> MAAPFDKSKNVAQSIDQLIGQTPALYLNKLNNTKAKVVLKMECENPMASVKDRLGFAIYDKAEKEGKLIPGKSIVVESSSGN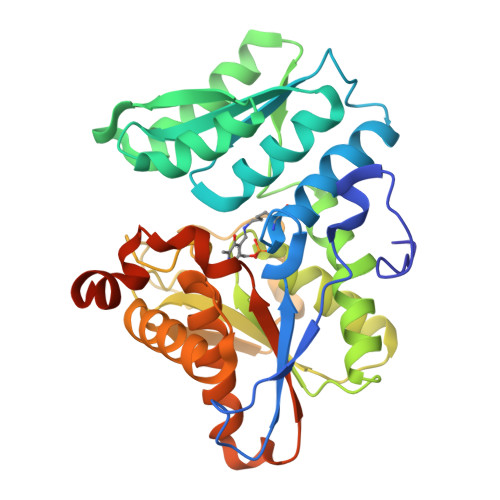TGVSLAHLGAIRGYKVIITMPESMSLERRCLLRIFGAEVILTPAALGMKGAVAMAKKIVAANPNAVLADQFATKYNALIHEETTGPEIWEQTNHNVDCFIAGVGTGGTLTGVARALKKMGSHARIVAVEPTESPVLSGGKPGPHKIQGIGPGFVPDVLDRSLIDEVLCVAGDDAIETALKLTRSDGVFCGFSGGANVYAALKIAERPEMEGKTIVTVIPSFGERYLSTTLYRSVRDEVSSLPVALEHHHHHH> AAYSYRPGPGAGPGPAAGAA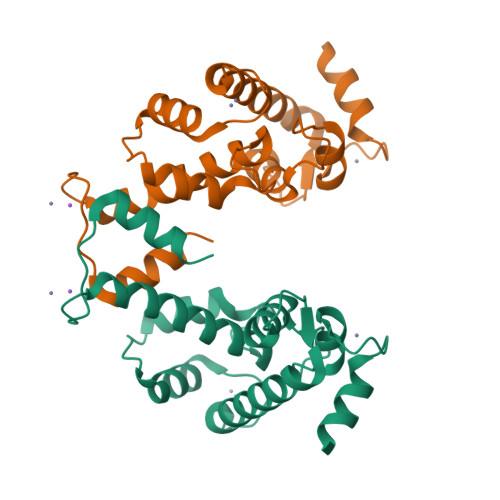LPDQSFLWNVFQRVDKDRSGVISDTELQQALSNGTWTPFNPVTVRSIISMFDRENKAGVNFSEFTGVWKYITDWQNVFRTYDRDNSGMIDKNELKQALSGFGYRLSDQFHDILIRKFDRQGRGQIAFDDFIQGCIVLQRLTDIFRRYDTDQDGWIQVSYEQYLSMVFSIV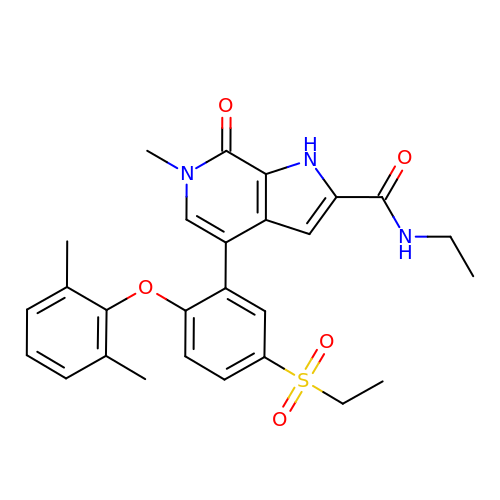4-[2-(2,6-dimethylphenoxy)-5-(ethylsulfonyl)phenyl]-N-ethyl-6-methyl-7-oxo-6,7-dihydro-1H-pyrrolo[2,3-c]pyridine-2-carboxamide | C27 H29 N3 O5 S | OPEBMJVHBSSVLY-UHFFFAOYSA-N>GPSSPSLLRAIPGIAWIALLLLVIFYVFAVMGTKLFAQSFPEWFGTLGASMYTLFQVMTLESWSMGIARPVIEAYPWAWIYFVSFILVSSFTVLNLFIGIIIESMQSAHWEAEDAKRIEQEQRAHDERLEMLQLIRDLSSKVDRLERRSGK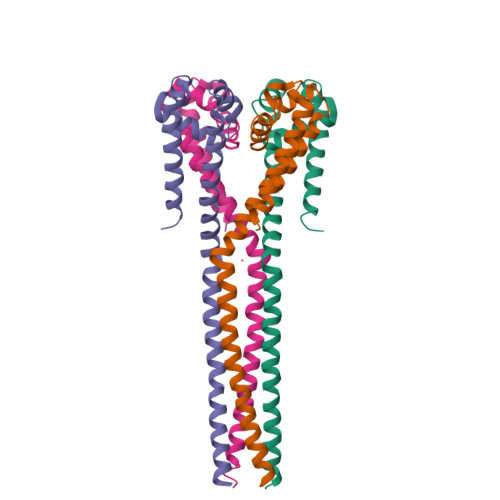R[4x]> TCNIKNGRCEQFCKNSADN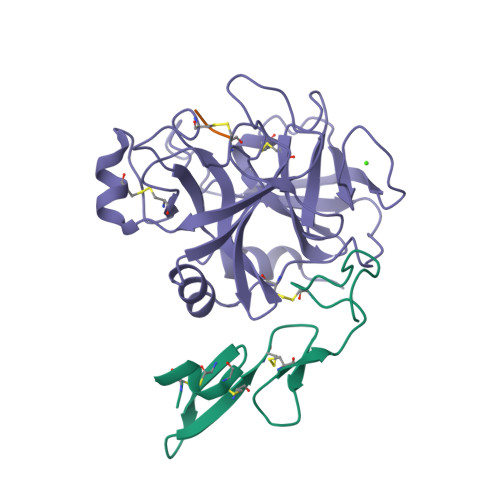KVVCSCTEGYRLAENQKSCEPAVPFPCGRVSVSQTSKLTR;> EGR;> VVGGEDAKPGQFPWQVVLNGKVDAFCGGSIVNEKWIVTAAHCVETGVKITVVAGEHNIEETEHTEQKRNVIRIIPHHNFNAAINTYNHDIALLELDEPLVLNSYVTPICIADKEYTNIFLKFGSGYVSGWGRVFHKGRAALVLQYLRVPLVDRATCLRSTKFTITNNMFCAGFHEGGRDSCQGDSGGPHVTEVEGTSFLTGIISWGEECAMKGKYGIYTKVSRYVNWIKEKTKLT>[16x]MKKFNIKSLTLLIVLLPLIVNANNIDSHLLEQNDIAKYVAQSDTVGSFFERFSALLNYPIVVSKQAAKKRISGEFDLSNPEEMLEKLTLLVGLIWYKDG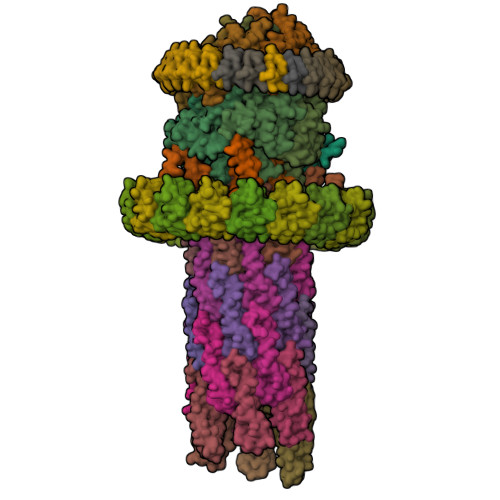NALYIYDSGELISKVILLENISLNYLIQYLKDANLYDHRYPIRGNISDKTFYISGPPALVELVANTATLLDKQVSSIGTDKVNFGVIKLKNTFVSDRTYNMRGEDIVIPGVATVVERLLNNGKALSNRQAQNDPMPPFNITQKVSEDSNDFSFSSVTNSSILEDVSLIAYPETNSILVKGNDQQIQIIRDIITQLDVAKRHIELSLWIIDIDKSELNNLGVNWQGTASFGDSFGASFNMSSSASISTLDGNKFIASVMALNQKKKANVVSRPVILTQENIPAIFDNNRTFYVSLVGERNSSLEHVTYGTLINVIPRFSSRGQIEMSLTIEDGTGNSQSNYNYNNENTSVLPEVGRTKISTIARVPQGKSLLIGGYTHETNSNEIISIPFLSSIPVIGNVFKYKTSNISNIVRVFLIQPREIKESSYYNTAEYKSLISEREIQKTTQIIPSETTLLEDEKSLVSYLNY;>MLSDMSLIATLSFFTLLPFLVAAGTCYIKFSIVFVMVRNALGLQQVPSNMTLNGIALIMALFVMKPIIEAGYENYLNGPQKFDTISDIVRFSDSGLMEYKQYLKKHTDLELARFFQRSEEENADLKSAENNDYSLFSLLPAYALSEIKDAFKIGFYLYLPFVVVDLVISSILLALGMMMMSPITISVPIKLVLFVALDGWGILSKALIEQYINIPA[5x];> MDISSWFESIHVFLILLNGVFFRLAPLFFFLPFLNNGIISPSIRIPVIFLVASGLITSGKVDIGSSVFEHVYFLMFKEIIVGLLLSFCLSLPFWIFHAVGSIIDNQRGATLSSSIDPANGVDTSELAKFFNLFSAVVFLYSGGMVFILESIQLSYNICPLFSQCSFRISNILTFLTLLASQAVILASPVMIVLLLSEVLLGVLSRFAPQMNAFSVSLTIKSLLAIFIIFICSSTIYFSKVQFFLGEHKFFTNLFVR;>MSDIVYMGNKALYLILIFSLWPVGIATVIGLSIGLLQTVTQLQEQTLPFGIKLIGVSISLLLLSGWYGEVLLSFCHEIMFLIKSGV[4x];> MANKTEKPTPKKLKDAAKKGQSFKFKDLTTVVIILVGTFTIISFFSLSDVMLLYRYVIINDFEINEGKYFFAVVIVFFKIIGFPLFFCVLSAVLPTLVQTKFVLATKAIKIDFSVLNPVKGLKKIFSIKTIKEFFKSILLLIILALTTYFFWINDRKIIFSQVFSSVDGLYLIWGRLFKDIILFFLAFSILVIILDFVIEFILYMKDMMMDKQEIKREYIEQEGHFETKSRRRELHIEILSEQTKSDIRNSKLVVMNPTHIAIGIYFNPEIAPAPFISLIETNQCALAVRKYANEVGIPTVRDVKLARKLYKTHTKYSFVDFEHLDEVLRLIVWLEQVENTH;>MNYIYPVNQVDIIKASDFQSQEISSLEDVVSAKYSDIKMDTDIQVSQIMEMVSNPESLNPESLAKLQTTLSNYSIGVSLAGTLARKTVSAVETLLKS[6x];>[28x]MASWSHPQFEKIEGRMSVTVPNDDWTLSSLSETFDDGTQTLQGELTLALDKLAKNPSNPQLLAEYQSKLSEYTLYRNAQSNTVKVIKDVDAAIIQNFR;>[24x]MIRYKGFILFLLLMLIGCEQREELISNLSQRQANEIISVLERHNITARKVDGGKQGISVQVEKGTFASAVDLMRMYDLPNPERVDISQMFPTDSLVSSPRAEKARLYSAIEQRLEQSLVSIGGVISAKIHVSYDLEEKNISSKPMHISVIAIYDSPKESELLVSNIKRFLKNTFSDVKYENISVILTPKEEYVYTNVQPVKEVKSEFLTNEVIYLFLGMAVLVVILLVWAFKTGWFKRNKI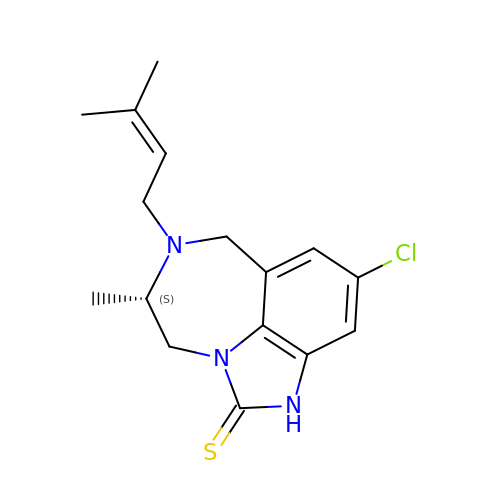4-CHLORO-8-METHYL-7-(3-METHYL-BUT-2-ENYL)-6,7,8,9-TETRAHYDRO-2H-2,7,9A-TRIAZA-BENZO[CD]AZULENE-1-THIONE | C16 H20 Cl N3 S | RCSLUNOLLUVOOG-NSHDSACASA-N(4S)-4-hydroxy-2-oxoheptanedioic acid | C7 H10 O6 | 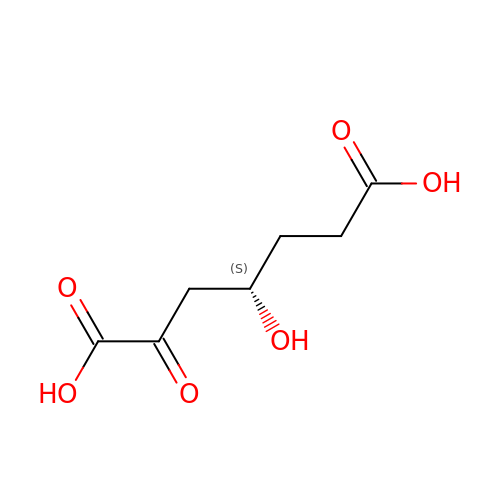HNOAJOYERZTSNK-BYPYZUCNSA-N> MIPALIETVIGCLLHDIGKPVQRAALGYRGRHSAIGRAFVKKIWLRDGRNPSEFADEVYEPDIEVFDRRILDAISYHHSSALRTAAENGRLAADAPAYVAYIADNIAAGTDRRKADSDDGQGASTWDSDTPLYSVFNRFGADTANLTFAPEMLDDREPMNIPSARRIEFDKYRYTEIVNKLEAVLVDLECSDTYLASLLNVLEATLSFVPSSTDASEVVDVSLFDHLKLTGALGACIWHYLQATGQSDFKSALFDKQDTFYNEKAFLLTTFDVSGIQDFIYTIHSSGAAKMLRARSFYLEMLTEHLIDELLARVGLSRANLNYSGGGHAYLLLPNTEFARNSLEEFEREANEWLLENFATWLFIATGSVPLAANDLMRRPNESGPQAHDRALRYSGLYRELSEQLSAKKLARYSADQLRELNSSDHDGQKGDRECSVCHTVNRTIKTINDLLLCSLCQALTAASQQIQSESRRFLLISEESSDGLPLPFGATLTFCSESGAKQALQQPQTRRLYAKNKFFAGESLGTGLWVGDYVAQMEFGDYVKRASGIARLGVLRLDVDNLGQAFTHGFMKQGNGKFNTISRTAAFSRMLSLFFRQHINYVLKHPKLRPLT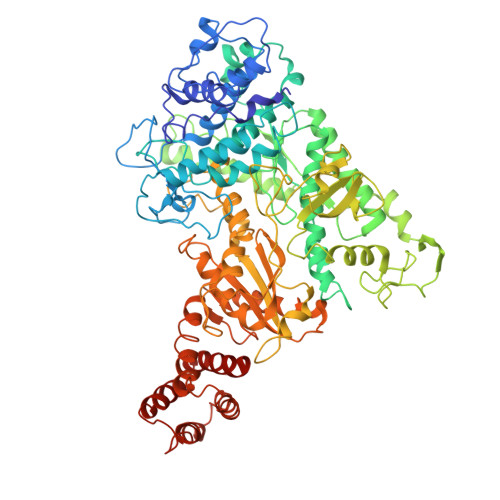GDDPERSRRATIIYSGGDDVFVVGAWDDVIEFGIELRERFHEFTQGKLTVSAGIGMFPDKYPISVMAREVGDLEGAAKSLPGKNGVALFDPEFTFRWDELLSKVIEEKYRHIADYFRCNEERGMAFIYKLLELLDQRGDRITEARWVYFLMRMRGPTDDTTRFQQFANRLHQWFQDPSDAKQLKTALHLYIYRNRKEESE> MASWDSPTASSNGDLIEEIQASSTSTDPRTFTGLSIVEDIGDVVPVTDNASPALPVSLTDADGNDVVVEDVSRILPLDLYGTYSKTIAGLGLVDNIVGRTVSSTEPALADTEVVTTGGATLNAEAILNLHPTLVIIDHSIGPRE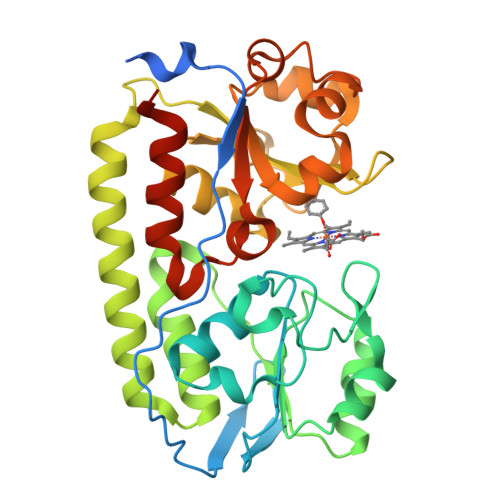VIDQIRAAGVATVIMSPQRSIASIGDDIRDIASVVGLPEEGEKLAERSVAEVEEASTVVDELTPEDPLKMVFLYARGTGGVFFILGDAYGGRDLIEGLGGVDMAAEKGIMDLAPANAEALAELNPDVFVMMSEGLVSTGGIDGLMERPGIAQTTAGQNQRVLALPDGQSLAFGAQTGELLLRASRELYVQGGELEHHHHHH> MDYKDDDDKMVLSQEEPDSARGTSEAQPLGPAPT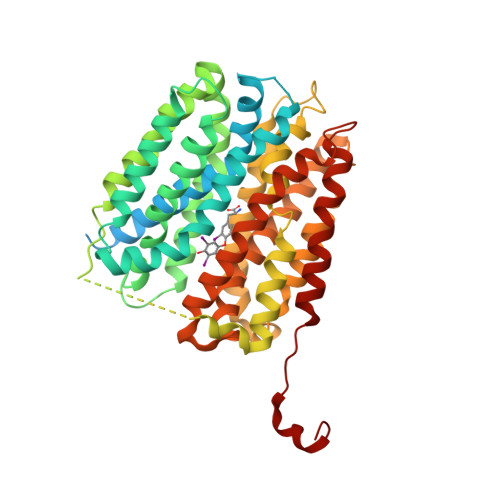GAAPPPGPGPSDSPEAAVEKVEVELAGPATAEPHEPPEPPEGGWGWLVMLAAMWCNGSVFGIQNACGVLFVSMLETFGSKDDDKMVFKTAWVGSLSMGMIFFCCPIVSVFTDLFGCRKTAVVGAAVGFVGLMSSSFVSSIEPLYLTYGIIFACGCSFAYQPSLVILGHYFKKRLGLVNGIVTAGSSVFTILLPLLLRVLIDSVGLFYTLRVLCIFMFVLFLAGFTYRPLATSTKDKESGGSGSSLFSRKKFSPPKKIFNFAIFKVTAYAVWAVGIPLALFGYFVPYVHLMKHVNERFQDEKNKEVVLMCIGVTSGVGRLLFGRIADYVPGVKKVYLQVLSFFFIGLMSMMIPLCSIFGALIAVCLIMGLFDGCFISIMAPIAFELVGAQDVSQAIGFLLGFMSIPMTVGPPIAGLLRDKLGSYDVAFYLAGVPPLIGGAVLCFIPSRLEEELRRRLTEP> MAAIQGIEGVISQLQATAMAARGQDTHS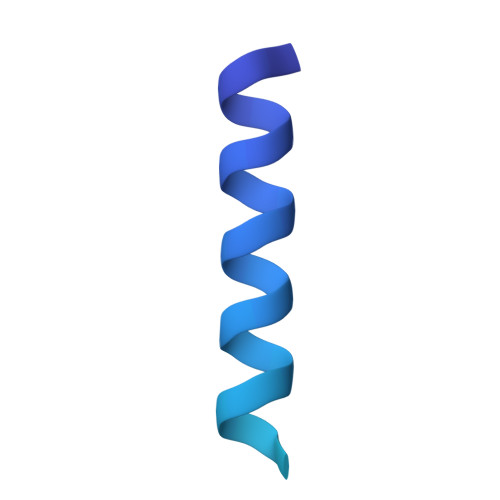QSTVSFAGQLHAALDRISDRQAAARVQAEKFTLGEPGIALNDVMADMQKASVSMQMGIQVRNKLVAAYQEVMSMQV Ferroportin (Fpn) activity plays a central role in human iron homeostasis on both systemic and cellular levels. In vertebrates, Fpn is subject to post-translational regulation by the hormone hepcidin, a key event in iron pathophysiology. Hepcidin binds to active Fpn and signals the endocytosis and proteolysis of the Fpn–hepcidin complex when systemic iron levels are high. Detailing the nature of the Ca2+ dependence, we present the crystal structure of a Ca2+-bound BbFpn protein, which supports a model in which Ca2+ is a required cofactor that facilitates a conformational change critical to the transport cycle.

To delineate the functional rationale for the Ca2+ dependence of Fpn, we obtained a new crystal form of BbFpn in the presence of CaCl2 and determined the structure at a resolution of 3.2 Å. The asymmetric unit consists of a single monomer comprised of 12 TM helices organized into two domains, as is typical of MFS transporters. The structure revealed an ion-binding site localized in the center of the N-terminal domain. We tentatively ascribed this site to Ca2+ based on the constituents of the crystallization condition, and hereafter refer to the structure as Ca2+-bound. All of the side-chain oxygen atoms, except for that of E203, are arranged on roughly the same plane along the membrane normal, whereas E203 forms an apparent bidentate coordination with Ca2+ from the intracellular side. Most prominently, the coordination of Ca2+ by N196 and E203 produces a distinct kink in the TM6 helix between these two residues, resulting in a marked displacement of E203—the carboxylate group is shifted by ∼5 Å. In the structure presented here, crystallized at pH 8, the presence of Ca2+ appears to be catalyzing the conformational change to the inward conformation. Upon examination of the Ca2+-bound BbFpn structure, we identified a proposed substrate-binding site in the C-terminal domain. However, this pocket was empty in the structures previously obtained for BbFpn. Unexpectedly, in the pocket of the new structure, we observed clear non-protein electron density, which we have unambiguously assigned to a Ni-EDTA complex carried through from the protein purification procedure. In the structure, the EDTA moiety is seated in a largely hydrophobic area formed by residues from TM7, TM10, TM11, and is hydrogen-bonded to the hydroxyl group of S256 and S259, carbonyl group of H261, and backbone amino groups of G262 and V263.

> MKVQSLLRIETQLLLGRLLTRSGDQAWDFVVPFALLVIFPGKLQVAAFYYLIVKIGTFLLTPSSGKWIDTHPRIQVVKWGVWLQFFAILAGMVFFGMLDGLVRAGGRESWLLSVLFIALALSGVMASLGSQITDISVGNDLAPSLVAPEKLTHFNSWLRRIDLATEVGAPILAGALFAFHPEQLPLAGLFLIGLWNLVSFVPEYFLLRNVIQRSGLKIKVLTEAQSWKDTFHINLRGSFSDPIFWLILSYALLWLSVLSPHGVLLAAYLKDEMRLPETEIGLFRGLGAVFGLISTVSFPYLVRRLGLISSSRWHLGFQGVTLGIAVTAFAMGSTASVYVFLGCILLSRVGLYGFSNGEFELRQRLIPEGRRGELNSLSSLTTTSATLILFSAGSLLPQTEDFKYLVYVSLAAVLLANVVFIKWSSRQGVVTSGSENLYFQ> MPSPTTVPVATAGRLAEPYIDPAAQVHAIASIIGDVRIAAGVRVAAGVSIRADEGAPFQVGKESILQEGAVIHGLEYGRVLGDDQADYSVWIGQRVAITHKALIHGPAYLGDDCFVGFRSTVFNARVGAGSVIMMHALVQDVEIPPGRYVPSGAIITTQ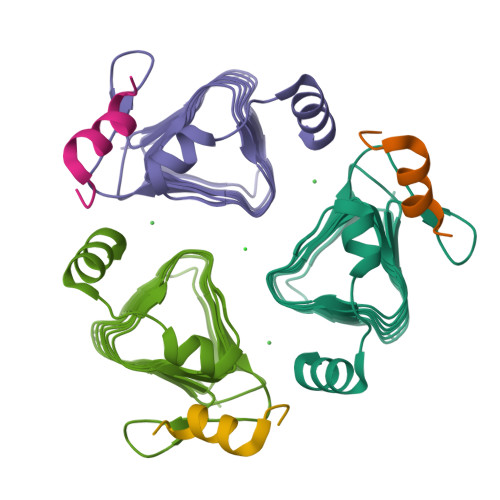QQADRLPEVRPEDREFARHIIG;> GWLAPEQQQRIYRGNAS> MGHHHHHHGSGSNRLDGKVAIITGGTLGIGLAIATKFVEEGAKVMITGRHSDVGEKAAKSVGTPDQIQFFQHDSSDEDGWTKLFDATEKAFGPVSTLVNNAGIAVNKSVEETTTAEWRKLLAVNLDGVFFGTRLGIKRMKNKGLGASIINMSSIEGFVGDPSLGAYNASKGAVRIMSKSAALDCALKDYDVRVNTVHPGYIKTPLVDDLPGAEEAMSQRTKTPMGHIGEPNDIAYICVYLASNES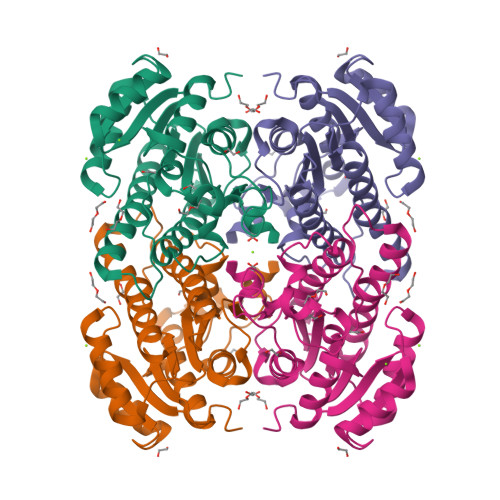KFATGSEFVVDGGYTAQ>MKKLLPILIGLSLTGFSAMSQAENLLQVYQQARISNPDLRKSAADRDAAFEKINEARSPLLPQLGLGADYTYTSGFRDYKDQNSNVTSGSLQLTQVLFDMSKWRALTLQEKAAGIQDVTYQTDQQTLILNTATAYFKVLAAIDTLSYTEAQKQAIYRQLDQTTQRFNVGLVAITDVQNARSQYDAVLANEVTARNDLDNAVEELRQVTGNYYPELASLNVDGFKTSKPQAVNALLKEAENRNLSLLQARLNQDLAREQIRQAQDGHLPTLDLNASSGVSNNRYSGSKSISQDADIGQNKIGLSFSLPLYQGGMVNSQVKQAQYNFVGASEQLESAHRSVVQTVRSSFNNVNASISSINAYKQAVVSAQSSLDAMEAGYSVGTRTIVDVLDATTTLYNAKQQLSNARYNYLINELNIKSA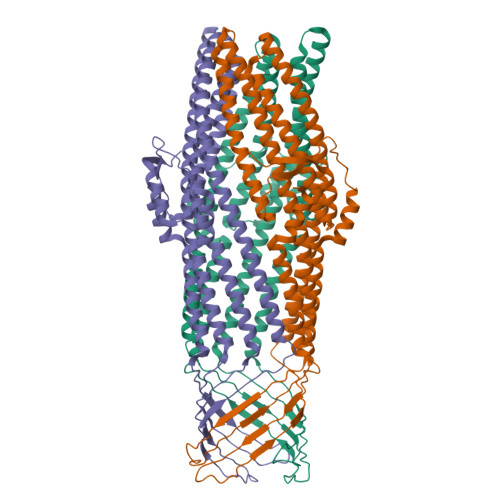LGTLNEQDLIALNNTLGKPISTSADSVAPENPQQDATADGYGNTTAAMKPASARTTTHSSGSNPFRQLEHHHHHH[3x]>[3x]PPAIGQFWHVTDLHLDPTYHITDDHTKVCASSKGANASNPGPFGDVLCDSPYQLILSAFDFIKNSGQEASFMIWT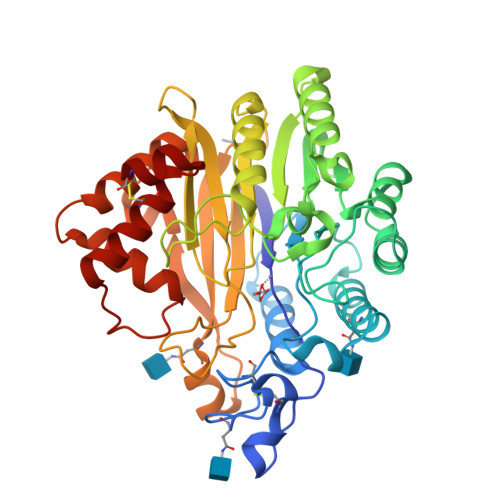GDSPPHVPVPELSTDTVINVITNMTTTIQSLFPNLQVFPALGNHDYWPQDQLPVVTSKVYNAVANLWKPWLDEEAISTLRKGGFYSQKVTTNPNLRIISLNTNLYYGPNIMTLNKTDPANQFEWLESTLNNSQQNKEKVYIIAHVPVGYLPSSQNITAMREYYNEKLIDIFQKYSDVIAGQFYGHTHRDSIMVLSDKKGSPVNSLFVAPAVTPVKSVLEKQTNNPGIRLFQYDPRDYKLLDMLQYYLNLTEANLKGESIWKLEYILTQTYDIEDLQPESLYGLAKQFTILDSKQFIKYYNYFFVSYDSSVTCDKTCKAFQICAIMNLDNISYADC> GSSDKGKLSLQDVAELIRARACQRVVVMVGAGISTPSGIPDFRSPGSGLYSNLQQYDLPYPEAIFELPFFFHNPKPFFTLAKELYPGNYKPNVTHYFLRLLHDKGLLLRLYTQNIDGLERVSGIPASKLVEAHGTFASATCTVCQRPFPGEDIRADVMADRVPRCPVCTGVVKPDIVFFGEPLPQRFLLHVVDFPMADLLLILGTSLEVEPFASLTEAVRSS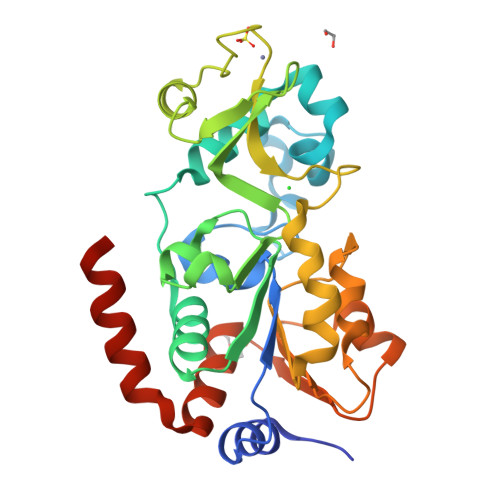VPRLLINRDLVGPLAWHPRSRDVAQLGDVVHGVESLVELLGWTEEMRDLVQRETGKLDGPDK;> TRSGKVMRRL> MHHHHHHLVFIDDGSTNIKLQWQESDGTIKQHISPNSFKREWAVSFGDKKVFNYTLNGEQYSFDPISPDAVVTTNIAWQYSDVNVVAVHHALLTSGLPVSEVDIVCTLPLTEYYDRNNQPNTENIERKKANFRKKITLNGGDTFTIKDVKVMPESIPAGYEVLQELDERDS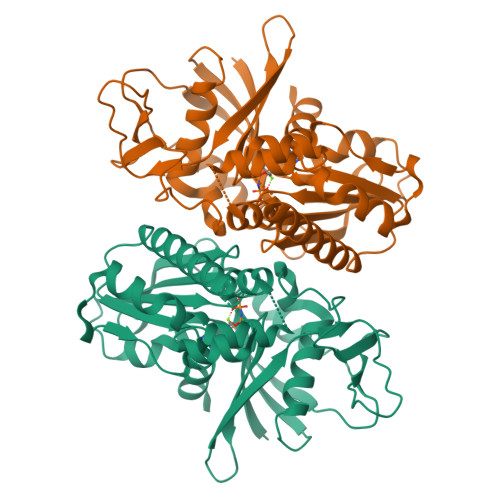LLIIDLGGTTLDISQVMGKLSGISKIYGDSSLGVSLVTSAVKDALSLARTKGSSYLADDIIIHRKDNNYLKQRINDENKISIVTEAMNEALRKLEQRVLNTLNEFSGYTHVMVIGGGAELICDAVKKHTQIRDERFFKTNNSQYDLVNGMYLIGN> GAPPAPALRIDYPKALQILTEGGTHMVCTGRTHTDRLCRFKWLCYSSEAEEFIFFHGNASVMLPSLGSRRFQPALLDLSTVEDHNTQYFNFVELPAAALRFMPKPVFVPDVALIANRFNPDNLMHVFHDDLLPLFYTLRQFPGLAREARLFFMEGWGEGAHFDLYKLLSPKQPLLRAQLKALGRLLCFSHAFVGLSKVTTWYQYGFVQPQGPKANILVSGNEIRQFAHFLMEKLNVSQAGGPLGEEYILVFSRTQNRLILNEAELLLALAQEFQMKTVTV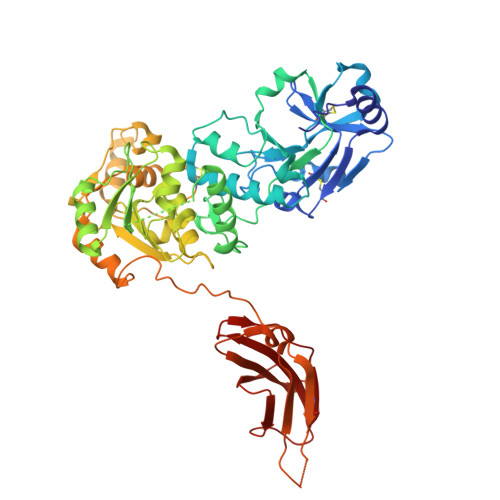SLEDHAFADVVRLVSNASMLVSMHGAQLVTALFLPRGAAVVELFPYAVNPDHYTPYKTLATLPGMDLQYIAWQNTMPENTVTHPERPWDQGGIAHLDRAEQARILQSREVPRHLCCRNPEWLFRIYQDTKVDIPSLIQTIRRVVKGHPGPRKQKWTVSLYPGKVREARCQASVQGASEARLSVSWQIPWNLKYLKVREVKYEVWLQEQGENTYVPYMLALQNHTFTENIKPFTTYLVWIRCIFNKTLLGPFADVLVCST(2,4-dinitrophenyl)-[4-[(4-fluorophenyl)methyl]piperazin-1-yl]methanone | C18 H17 F N4 O5 | 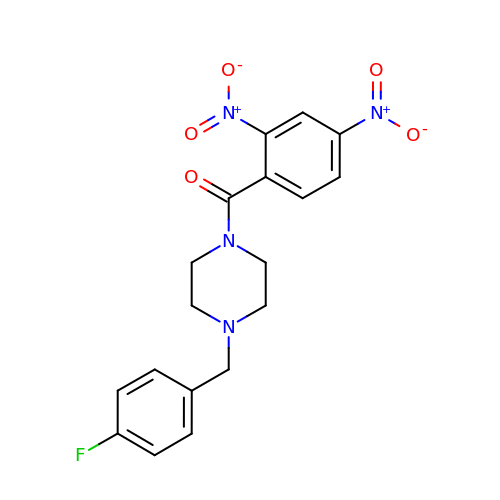ZPXJBWPENHAIHH-UHFFFAOYSA-N N1-FORMYL-TRYPTOPHAN | C12 H12 N2 O3 | 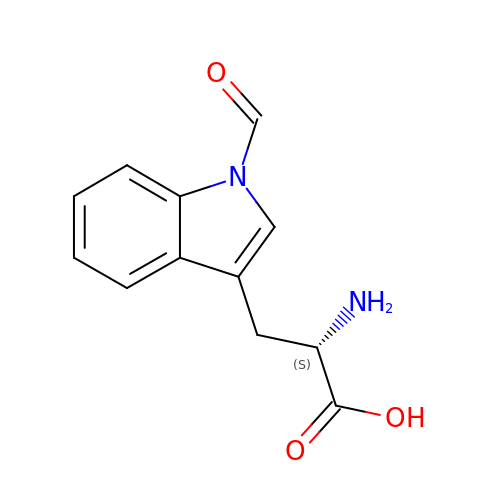KRUDZOGZZBVSHD-JTQLQIEISA-N>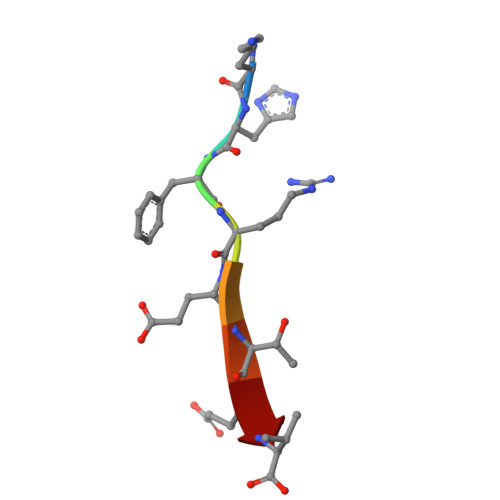 KHFRETEV>MSLTLRLAEHRDLEAVVAIYNSTIASRMVTADTEPVTPEDRMEWFSGHTESRPLYVAEDENGNVAAWISFETFY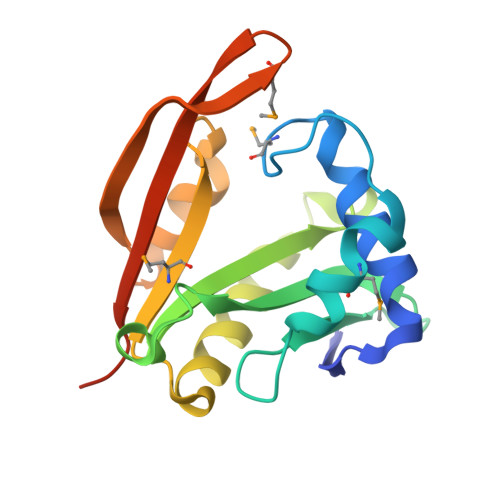GRPAYNKTAEVSIYIDEACRGKGVGSYLLQEALRIAPNLGIRSLMAFIFGHNKPSLKLFEKHGFAEWGLFPGIAEMDGKRYDLKILGRELSEGGSHHHHHH[2x]> ADYQGKNVVIIGLGLTGLSCVDFFLARGVTPRVMDTRMTPPGLDKLPEAVERHTGSLNDEWLMAADLIVASPGIALAHPSLSAAADAGIEIVGDIELFCREAQAPIVAITGSNGKSTVTTLVGEMAKAAGVNVGVGGNIGLPALMLLDDECELYVLELSSFQLETTSSLQAVAATILNVTEDHMDRYPFGLQQYRAAKLRIYENAKVCVVNADDALTMPIRGADERCVSFGVNMGDYHLNHQQGETWLRVKGEKVLNVKEMKLSGQHNYTNALAALALADAAGLPRASSLKALTTFTGLPHRFEVVLEHNGVRWINDSKATNVGSTEAALNGLHVDGTLHLLLGGDGKSADFSPLARYLNGDNVRLYCFGRDGAQLAALRPEVAEQTETMEQAMRLLAPRVQPGDMVLLSPACASLDQFKNFEQRGNE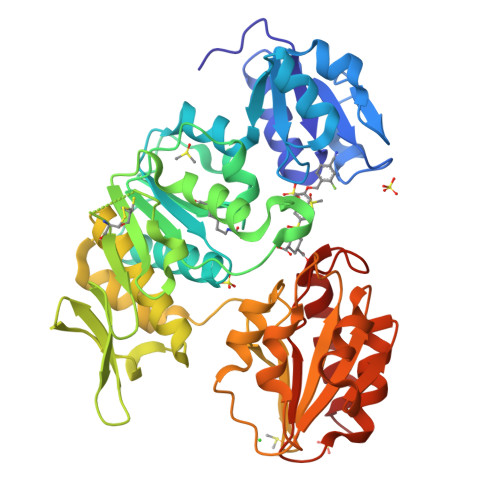FARLAKELGSH> MLAGVKKDIEKLYEAVPQLSNVFKIEDKIGEGTFSSVYLATAQLQVGPEEKIALKHLIPTSHPIRIAAELQCLTVAGGQDNVMGVKYCFRKNDHVVIAMPYLEHESFLDILNSLSFQEVREYMLNLFKALKRIHQFGIVHRDVKPSNFLYNRRLKKYALVDFGLAQGTHDTKIELLKFVQSEAQQERCSQNKCSICLSRRQQVAPRAGTPGFRAPEVLTKCPNQTTAIDMWSAGVIFLSLLSGRYPFYKASDDLTALAQIMTIRGSRETIQAAKTFGKSILCSKEVPAQDLRKLCERLRGM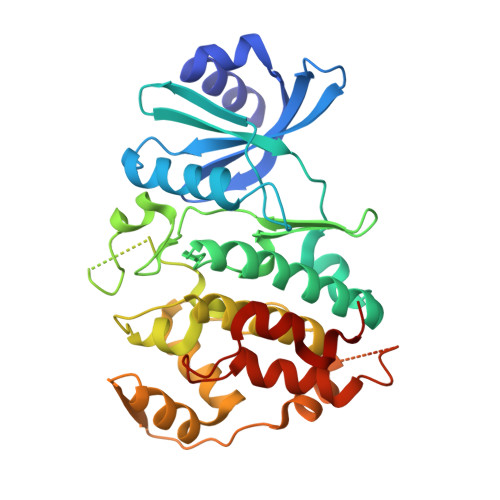DSSTPKLTSDIQGHATNLEGWNEVPDEAYDLLDKLLDLNPASRITAEEALLHPFFKDMSL> GHMREIADKLIELKAEIEELQQREQELDQHKVWVQQSIRNVTEDVQNSCLAYVTH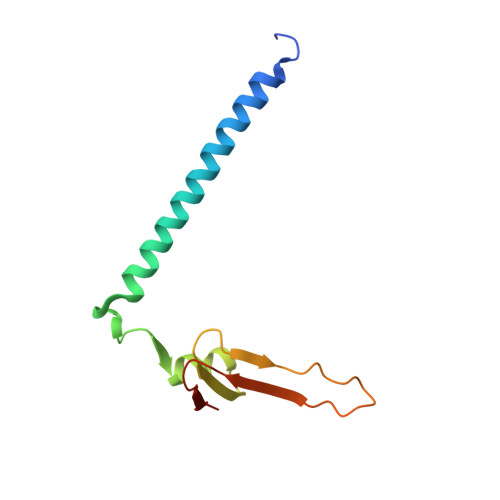EDICRCFAGDTLLAIRAPSGTSLEVPIPEGLNGQKKYQIHLKSVSGPIEVLLVNKE> MGAQV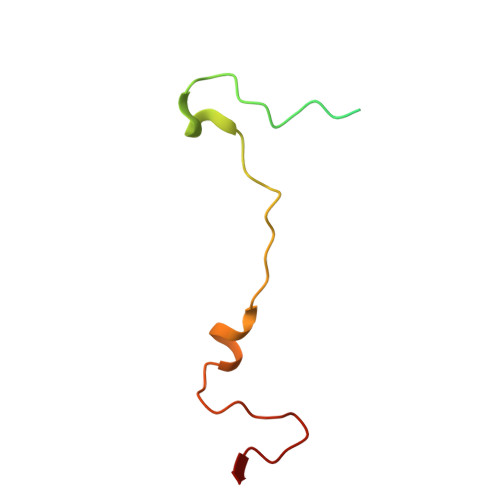STQKSGSHETRNVATEGSTINFTNINYYKDSYAASASRQDFAQDPAKFTRPVLDAIREAAAPLQ> MFENITAAPADPILGLADLFRADERPGKINLGQGVYKDETGKTPVLTSVKKAEQYLLENETTKNYLGIDGIPEFGRCTQELLFGKGSALINDKRARTAQTPGGTGALRVAADFLAKNTSVKRVWVSNPSWPNHKSVFNSAGLEVREYAYYDAENHTLDFDALINSLNEAQAGDVVLFHGCCHNPTGIDPTLEQWQTLAQLSVEKGWLPLFDFAQQGFARGLEEDAEGLRAFAAMHKELIVASSYSKNFGLYNERVGACTLVAADSETVDRAFSQMKAAIYANYSNPPAHGASVVATILSNDALRAIWEQELTDMRQRIQRMRQLFVNTLQEKGANRDFSFIIKQNGMFSFSGL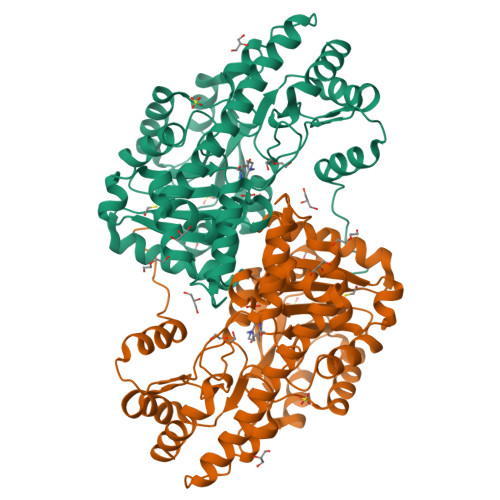TKEQVLRLREEFGVYAVASGRVNVAGMTPDNMAPLCEAIVAVL N-[(2S)-2-amino-2-carboxyethyl]-L-glutamic acid | C8 H14 N2 O6 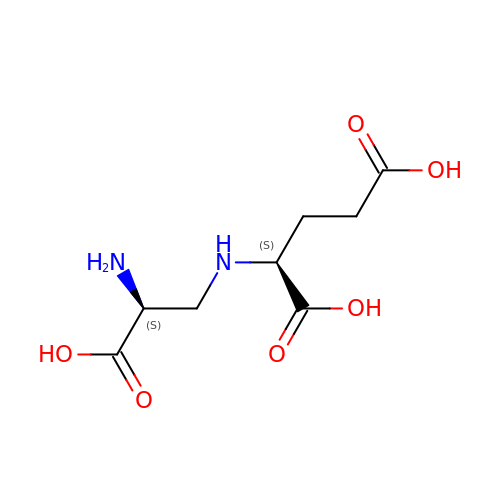| XYQHCOGLGSNTNV-WHFBIAKZSA-N> NHTNVKFLFDRSRLLNVIKVLEKDAVFPRPFPTATGTQQDDGYFCLLTPRPTVASRPATRFGLYVSPSDSGVLANTSLDFNFYSLACFTYFRSDLEVTVVSLEPDLEFAVGWFPSGSEYQASSFVYDQLHVPYHFTGRTPRAFASKGGKVSFVLPWNSVSSVLPVRWGGA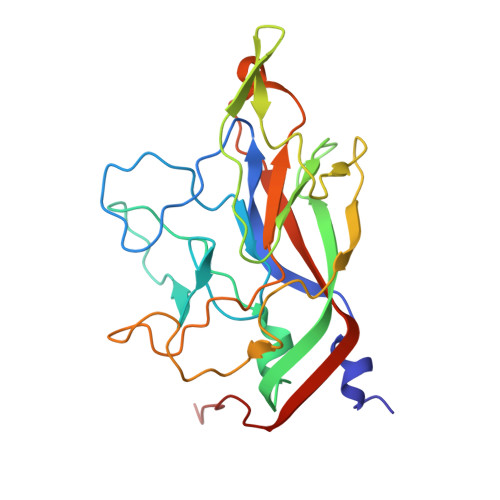SKLSSATRGLPAHADWGTIYAFIPRPNEKKSTAVKHVAVYIRYKNARAWCPSMLPFRSYK>[2x]DVSGT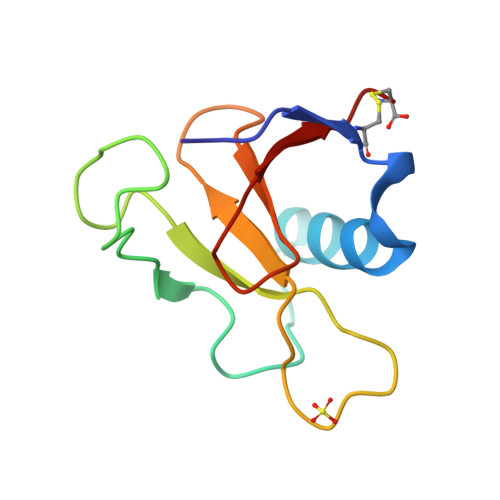VCLSALPPEATDTLNLIASDGPFPYSQDGVVFQNRESVLPTQSYGYYHEYTVITPGARTRGTRRIITGEATQEDYYTGDHFATFSLIDQTC> MPALDLIRPSVTAMRVIASVNADFARELKLPPHIRSLGLISADSDDVTYIAADEATKQAMVEVVYGRSLYAGAAHGPSPTAGEVLIMLGGPNPAEVRAGLDAMIAHIENGAAFQWANDAQDTAFLAHVVSRTGSYLSSTAGITLGDPMAYLVAPPLEATYGIDAALKSADVQLATYVPPPSETNYSAAFLTGSQAAC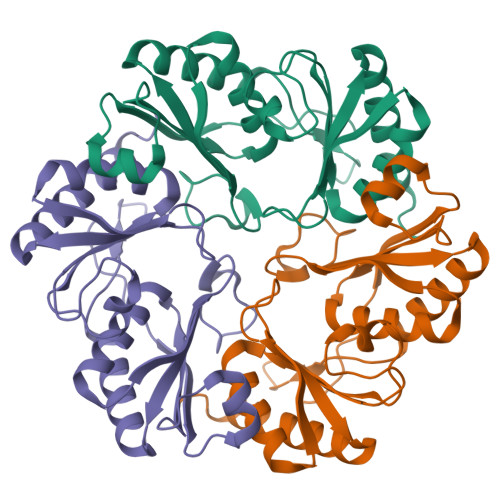KAACNAFTDAVLEIARNPIQRALEHHHHHH> GSMASGGPCCSHARIPRTPYLVLSYVN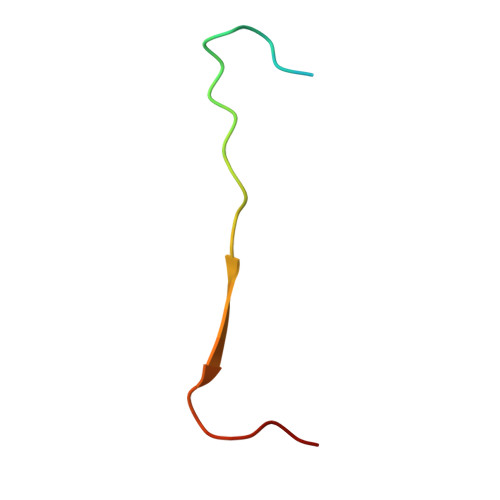GLPPV> MHHHHHHHTGAAPDRKAPVRPTPLDRVIPAPASVDPGGAPYRITRGTHIRVDDSREARRVGDYLADLLRPATGYRLPVTAHGHGGIRLRLAGGPYGDEGYRLDSGPAGVTITARKAAGLFHGVQTLRQLLPPAVEKDSAQPGPWLVAGGTIEDTPRYAWRSAMLDVSRHFFGVDEVKRYIDRVARYKYNKLHLHLSDDQGWRIAIDSW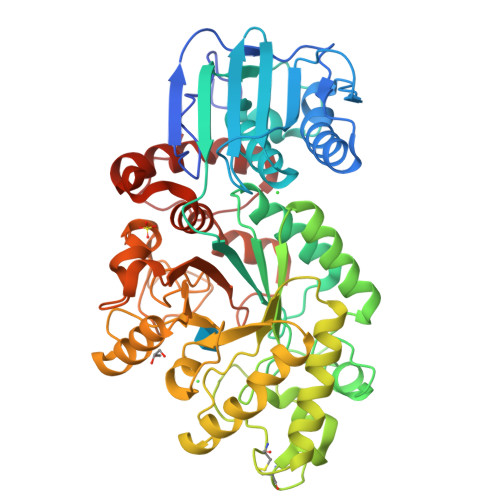PRLATYGGSTEVGGGPGGYYTKAEYKEIVRYAASRHLEVVPEIDMPGHTNAALASYAELNCDGVAPPLYTGTKVGFSSLCVDKDVTYDFVDDVIGELAALTPGRYLHIGGNEAHSTPKADFVAFMKRVQPIVAKYGKTVVGWHQLAGAEPVEGALVQYWGLDRTGDAEKAEVAEAARNGTGLILSPADRTYLDMKYTKDTPLGLSWAGYVEVQRSYDWDPAGYLPGAPADAVRGVEAPLWTETLSDPDQLDYMAFPRLPGVAELGWSPASTHDWDTYKVRLAAQAPYWEAAGIDFYRSPQVPWT> 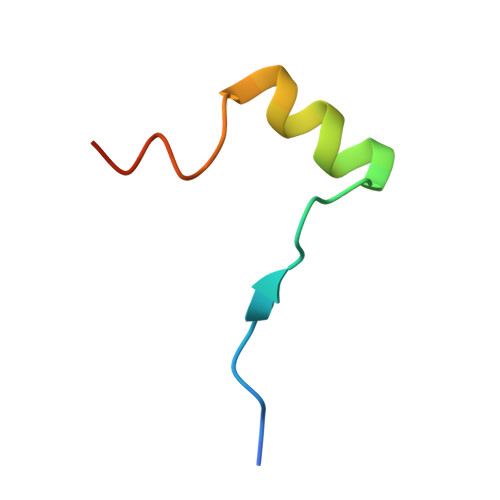SPLFAEPYKVTSKEDYLSSRIQSMLGNYDEMKDFIG> GRSEKQKQVIPVVNPTLPQNFYEKPAFDYPMNQMSVWLMLANEGMAKNDSFCATTPSAMVFGKSDGDRFAVTRDLTLKPGYVLQFKLNIGCTSQFSSTAPVLLQYSHDAGMSWFLVKEGCFPASAGKGCEGNSRELSEPTVYYTGDFEEWTRITIAIPRSLASSKTRFRWIQESSSQKNVPPFGLDGVYISEPCPSYCSGHGDCISGVCFCDLGYTAAQGTCVSNTPNHSEMFDRFEGKLSPLWYKITGGQVGTGCGTLNDGRSLYFNGLGKREARTVPLDTRNIRLVQFYIQIGSKTSGITCIKPRARNEGLVVQY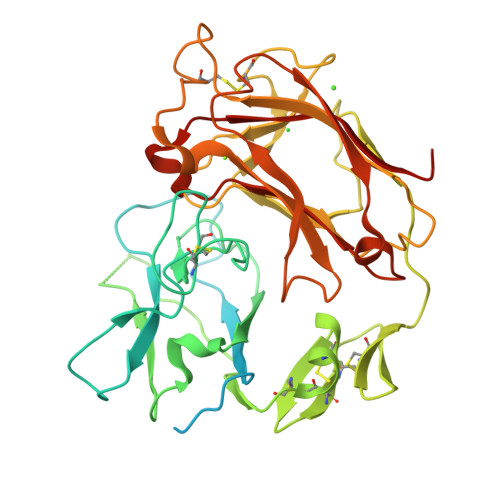SNDNGILWHLLRELDFMSFLEPQIISIDLPREAKTPATAFRWWQPQHGKHSAQWALDDVLISRLENLYFQ> GCPRILIRCKQDSDCLAGCVCTNNKFCGSPHHHHH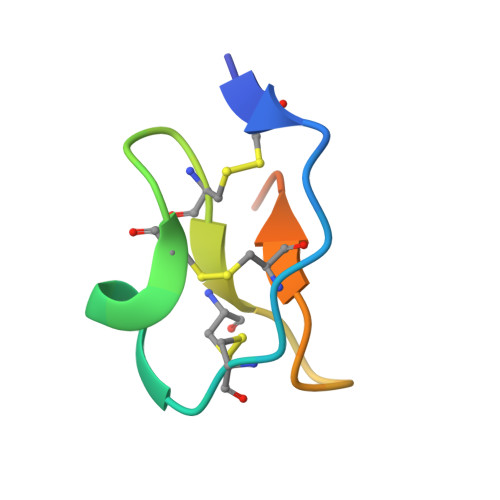H> MASHTADADAKPDSDSQKLLNVLPVSLRLRTRPWWFPIQEVSNPLVLYMEAWVAERVIGTDQAEISEIEWMCQALLTVDSVNSGNLAEITIFGQPSAQTRMKNILLNMAAWHKENELQRAVKVKEVEEFLK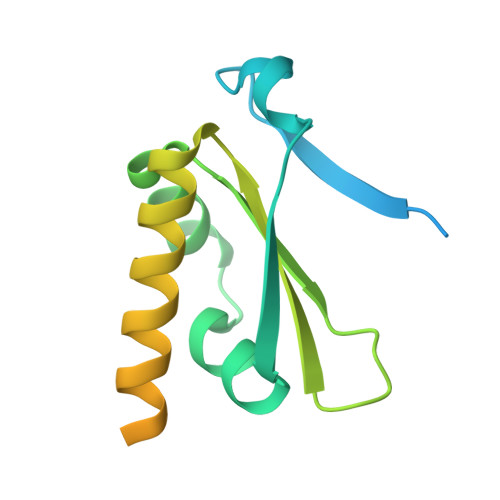IRASSILSKLSKKGLKLAGFPLPLEGRETQMES> EESYKR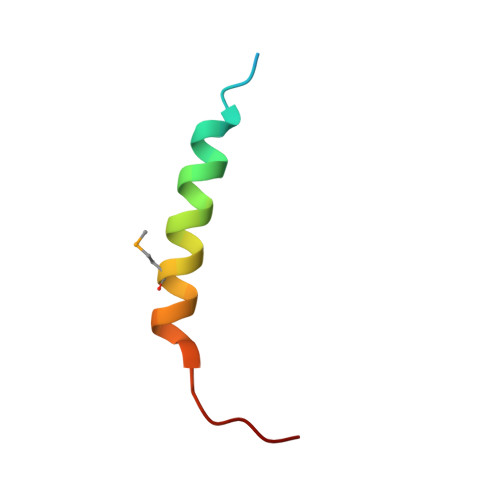AAAVTSTLKARIEKMKAKSRREGTTRT5-[ethyl(methyl)amino]-~{N}-[6-[[(1~{S},2~{R},3~{S},4~{R})-2-(hydroxymethyl)-3,4-bis(oxidanyl)cyclopentyl]amino]hexyl]naphthalene-1-sulfonamide 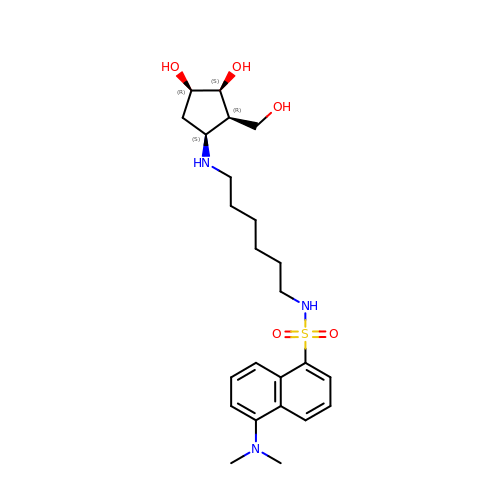| C24 H37 N3 O5 S | YQJKLKLPVRSCCE-QRVLJTFESA-N> MVIIMPGTKQVNVGSLKVGQ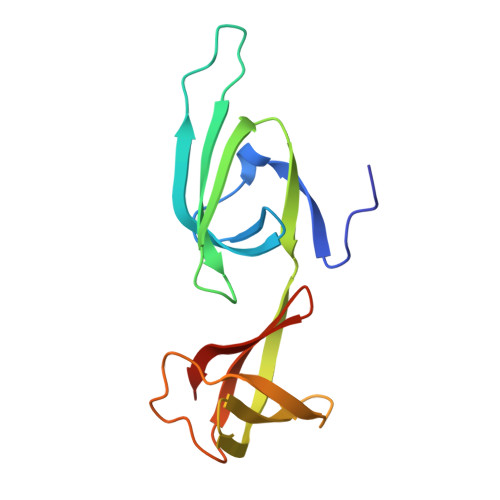YVMIDGVPCEIVDISVSKPGKHGGAKARVVGIGIFEKVKKEFVAPTSSKVEVPIIDRRKGQVLAIMGDMVQIMDLQTYETLELPIPEGIEGLEPGGEVEYIEAVGQYKITRVIGGK>[3x]XGEIAQGI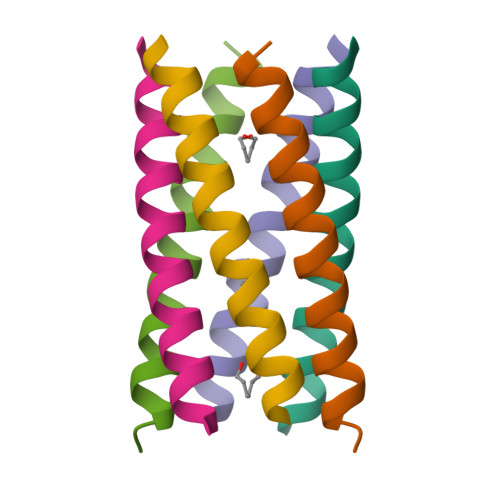KEIAKGIKEIAWGIKEIAQGIKGX>AHMMEKLKEIEKVTKAIKEKILNHYGYIRVITHHDTDGLSSGGILAKMLMRTNKLFHLTVVEHLSKEVIEKLAKENEVNKPLFIFAAMGSGQIEEIIKHNFNAIILDHHPPVIKDSFINENIIQLNPHIFGVDGSREITASGVCYLVAREFGYYDLSVLAIVGIIGDMQYNPLLGLNKFIVNEAREYRYVKIMNDIVYNIYDVEIYKAIAYCTKPYIPDLASEGKAFKFLKDIGIDPNKKQLDDTDKKKLLSAIIFKYPKIENLLIDRYLIEHKVRDAFLLSEMLNAVGRNGLFAVGIGICLEDDECIKIGNQILWE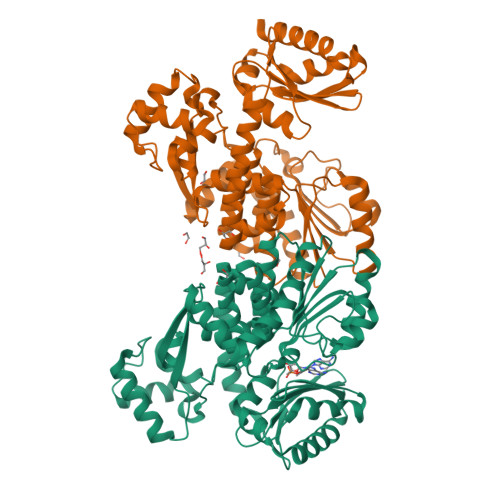YKKNLINELKSVKLKKLNNIYYFEGKKGMIGIIASILVDDKPVIGYHIEGDIAKFSARGNRDLVNRGLNLSVAMAVAKEFGGNGGGHDVASGAVVSKDKVQEFLKRVDEIIGEQLRR[2x]>HMYYSYGNYEAFARPKKPENVENKSAYLIGSGLASLAAACFLIRDGQMEGSKIHILEELPKAGGSLDGENMPLKGYVVRGGREMENHFECLWDLFRSIPSLEIDNASVLDEFYWLNKEDPNYSRCRVIEKQGQRLVTDGDFTLTKTAIKEIVDLCLTNEEDLDDVKITDVFSDDFFNSNFWIYWKTMFAFEPWHSAMEMRRYLMRFVHHISGLADFSALKFTKYNQYESLVLPMVEYLKSHGVQFEYDVKVEDIKIDVTTSQKIAREILIDRNGNAESIKLTINDLVFVTNGSITESSTYGDNDTPAPPTDELGGSWTLWKNLARQSPEFGNPDKFCQNIPKKSWFVSATSTTNNKEIIDTIESICKRDPLAGKTVTGGIITINDSAWQMSFTINRQQQFKDQPENEISTWIYALYSDVNGDYIKKPITECSGNEICQEWLYHLGVSTDKIEDLAKHASNTIPVYMPYITSYFMTRAIGDRPLVVPHQSQNLAFIGNFAETERDTVFTTEYSVRTAMEAVYQLLNIDRGIPEVINSPFDLRVLMDAIYELNDHQDLREITKDSKMQKLALAGF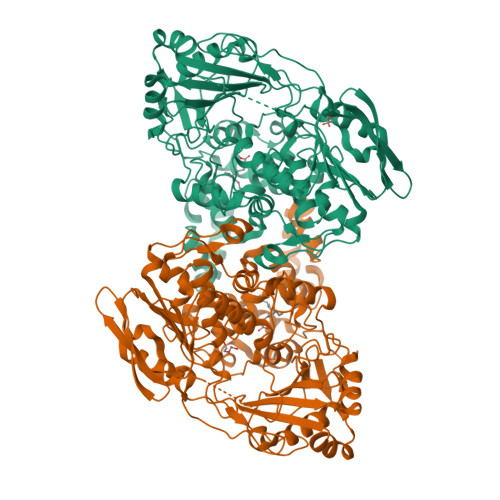LKKIKGTYIESLLKEHKLL[3x]> TNYLFSPNG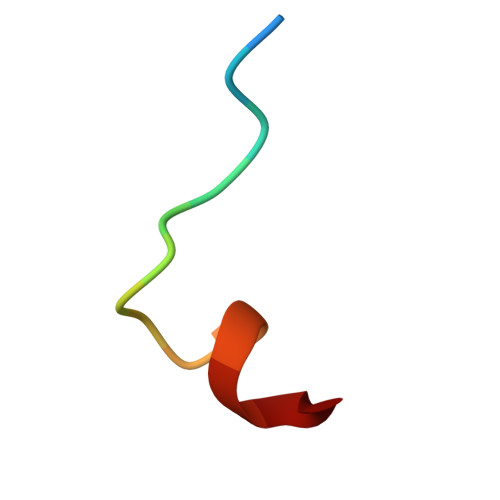PIARAW> IEALVPAWDSDIIFKCLCYFHTLYPGLIPLETFPPATIFNFKQKIISILEDKKAVLRGEPIKGPLPICCSKENYRRHLQRTTLLPVFMWYHPTPKTLSDTMQTMKQLAIKGSVGASHWLLVIVDIQARRLVYFDSLYNYVMPPENMKKELQSFAQQLDQVYPAYDSKKFSVKIAAKEVIQRGSGSSCGAWCCQFLHWYLKDPLTDALNDLPVDSVERHENLASFVQACEAAVQDLPELSWPEA;> GPRRQTIEALVPAWDSDIIFKCLCYFHTLYPGLIPLETFPPATIFNFKQKIISILEDKKAVLRGEPIKGPLPICCSKENYRRHLQRTTLLPVFMWYHPTPKTLSDTMQTMKQLAIKGSVGASHWLLVIVDIQARRLVYFDSLYNYVMPPENMKKELQSFAQQLDQVYPAYDSKKFSVKIAAKEVIQRGSGSSCGAWCCQFLHWYLKDPLTDALNDLPVDSVERHENLASFVQACEAAVQDLPELSWPEA

The chlamydial effector proteins ChlaDUB1 (CTL0247) and ChlaDUB2 (CTL0246), in the following termed Cdu1 and Cdu2, were demonstrated to have in vitro deubiquitinating and deneddylating activity. Sequence alignments clearly allocate Cdu1 into the family C48 of the CE clan of cysteine proteases. C. trachomatis Cdu1 is a 401 amino acid protein with a single-pass transmembrane domain located towards the N-terminus and a predicted flexible area up to residue 167. We further show that Cdu1 specifically deubiquitinates the major apoptosis regulator Mcl-1 at the surface of the inclusion.

In situ proteolysis and LCMS analysis identified a stable Cdu1 construct that displayed full proteolytic activity to pursue its structural characterization. The Cdu1 (155-401) fragment crystallized in space group P21 with two molecules in the asymmetric unit and at a resolution of 1.7 Å. Each monomer is composed of a central four-stranded β-sheet, which is surrounded by eight α-helixes resembling the architecture of the C48 proteases. The catalytic cysteine, Cys345, is located at the N-terminus of α-helix F, which is ‘sandwiched’ in between a set of three anti-parallel β-strands (1,2,3) and two extra α-helices, A and G, which are perpendicular to each other. β-strands 2 and 3 also contain the two other residues of the catalytic triad, His275 and Asp292. A search for other related structures utilizing the program DALI indicated that Cdu1 (155-401) shares a high degree of structural similarity with Ulp1 despite the fact that they only share 17% sequence identity within a stretch of 221 amino acids. Remarkably, however, a small loop between β-strands 1 and 2 (shown in yellow) in Ulp1 contrasts with the much bigger α-helix D in Cdu1 in between the equivalent β-strands of both structures. In contrast to this difference, the residues within the active site are highly conserved, further supporting the notion that Cdu1 forms a complex with ubiquitin in a similar way as observed between SENP8 and Nedd8 or Ulp1 and SMT3, respectively. The additional α-helix D in Cdu1, a feature not observed in the other structures, however, may play a regulatory role in substrate binding or recognition. Importantly, an insertion of identical length as observed in Cdu1 seems to be present in the Cdu1 proteins encoded by the genomes of C. suis, C. muridarum, C. psittaci, C. gallinaceai and Cdu2 from C. trachomatis suggesting that it is a conserved feature across the chlamydial deubiquitinases. We speculate that this helix could act like a ‘lid’ that plays a role in substrate binding and/or recognition and assumes a different orientation when the substrate is bound.>[2x]AVPGF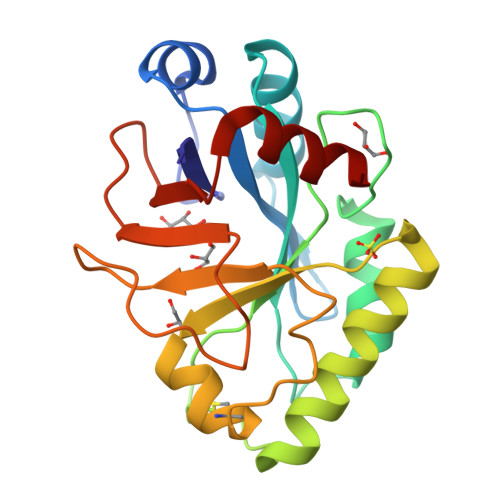DISHYQPSVNYAGAYNSGARFVIIKATEGTTYTDPVFSTHYTGATKAGLIRGGYHFARPASSSGSAQADFFFKNGGGWSADGITLPGMLDMEYGSTSSCHGLSQTAMVNWISDFVNRYKTLSGRYPMIYTGYYWWVECTGNSNKFATTCPLVLARYSSSVGEIPGGWGYQTIWQFNDKYAYGGDSDSFNGSLDRLKALAKGT>MICSVTGKPVKDVLSTFFKDRNDVLESEVKKFHLLATFEECKALAADTARRMNEYYKDVAEPVTLVALLTGAYLYASLLTVHLTFPYTLHFVKVSSYKGTRQESVVFDEEDLKQLKEKREVVLIDEYVDSGHTIF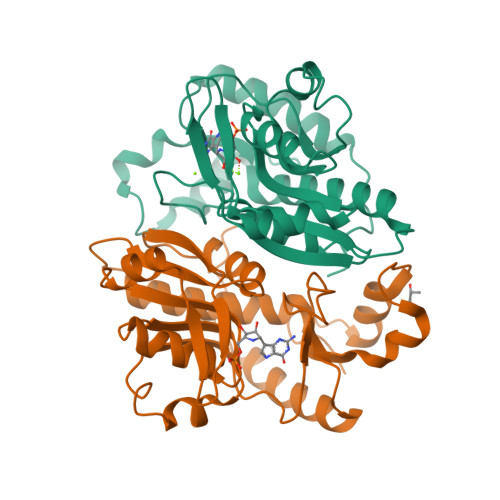SIQEQIKHAKICSCFVKDVDAIKKHSALADTKMFYGYTPMPKGSWLIGFGLDDNGLRRGWAHLFDINLSESEVTEFRRRLTEHIKGLNINGVNRY[2x]>[2x]GMTIQDYMLETPVRMREIISNADSLFNEVKRTNLKKIIITGSGTSYHSGVQVQPYLQNLLDIDVVKMYPFMITEDTFKFDNENTLVVGVSQGGSSYSTYNAMKLAEDKGCKIASMAGCKNALIDEISDYILTVNCGEEKSGAKTKGYYCTKLNLMLLGLQIAREKGIISSEKYNEEINKILDAINRFEAVYKLSKQWIERNKEKLVNSKEIRIIGHSDIY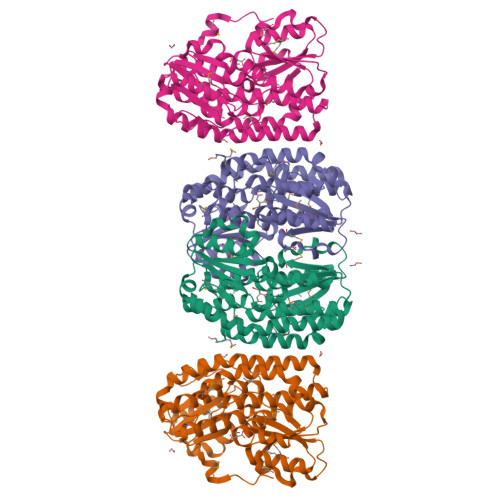GDTLEAALKLLETMRIPVTGYEFEEFIHGIYNAINSDSTIFILDTGKEPRVTKMIDVLSGWTENVFAIGRDVTENDKNLKIDITDNPYYQTFNFIVPIQLICGEIPTLRGVDPSVPKDTRFHMKLGSKKLNK> MACTIQRPEPQALRDKIATRFSTNVLGGAEIIPESNEFYVVTLEYAMQEEFFAFAEQMWREQDPRYACCENLVKMAARRGVYPKPAQFAQGYVRMTGVPGSALNQNLRFQFENQTYEAASVVPDQLPATGVLVLRVSAVTPGPSGNIRVTEGSLVTPVPGISSAVTAYGGNFCGGDDAEECEPFRTRYLQRLQYEPRLTVEWLKSKAMEWPCVTDVFDLGPNCCSVNALGEVECPNNIEFYVLFRDTFDCGLAPQCVVDEITDWLFGSPQGLGQGEAEFGICGKVRTATAVNLDIYLNGLSCATPAQARVVEQRITDFINRHPPSTNLTVEQLRFIGLQVLGSSFAFDVAI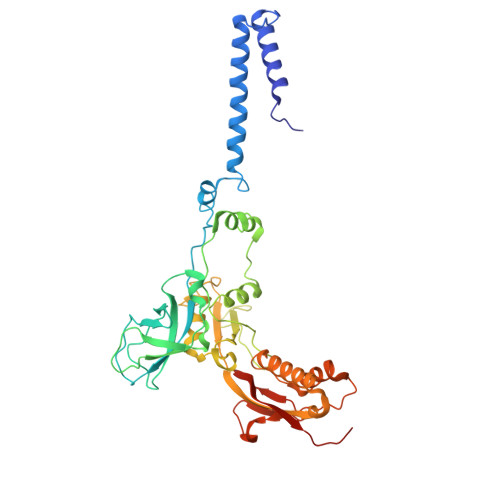RSPGDASQSGLRFNACGDAEIDCDYKACLNSVQVINNNVTTSGCL>ENLYFQSMRILVTGGSGLVGKAIQKVVADGAGLPGEDWVFVSSKDADLTDTAQTRALFEKVQPTHVIHLAAMVGGLFRNIKYNLDFWRKNVHMNDNVLHSAFEVGARKVVSCLSTCIFPDKTTYPIDETMIHNGPPHNSNFGYSYAKRMIDVQNRAYFQQYGCTFTAVIPTNVFGPHDNFNIEDGHVLPGLIHKVHLAKSSGSALTVWGTGNPRRQFIYSLDLAQLFIWVLREYNEVEPIILSVGEEDEVSIKEAAEAVVEAMDFHGEVTFDTTKSDGQFKKTASNSKLRTYLPDFRF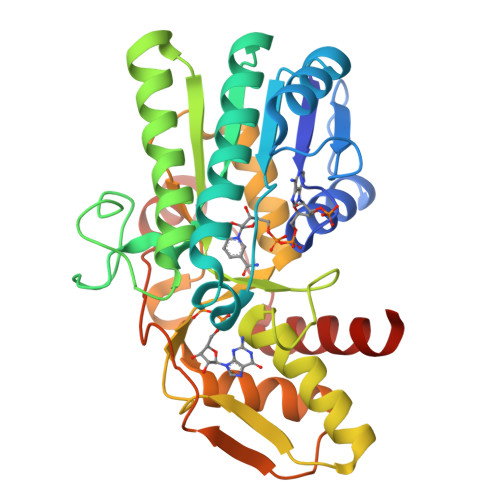TPFKQAVKETCAWFTDNYEQAR[4x]>SNASTTKLHPLINQKFQSPLSKEIFFESYFSTENLPFLADHIVYEQVVVPGASHISLLLAAASLTFAATECQIEDILFPQALAIPEQGVRTVQVVLTPQNNSFSFQVISFDDSLESQINQVSNNGSHISDWAVHATGKLSVANAEQSLIPLEEIQARC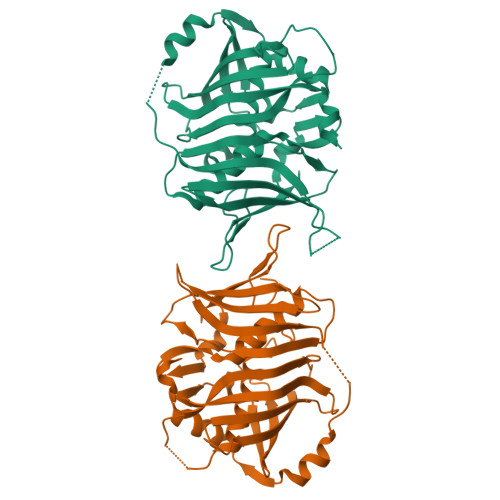SQKIDSAEIYQHLWDRQIHLGQSFRWIEQVWLGEGEVLCQMKVPKTILNTTKYQLHPTLVDSCFQSIIALVLDQSGNKNETFVPFSIDKFTFYNSSDNDLLWCYTCGSKDKQSGEKFKADIQLFDQHGQLVAQVIGFEGRKANPKILLMT[2x]> MAFSRPGLPVEYLQVPSASMGRDIKVQFQGGGPHAVYLLDGLRAQDDYNGWDINTPAFEE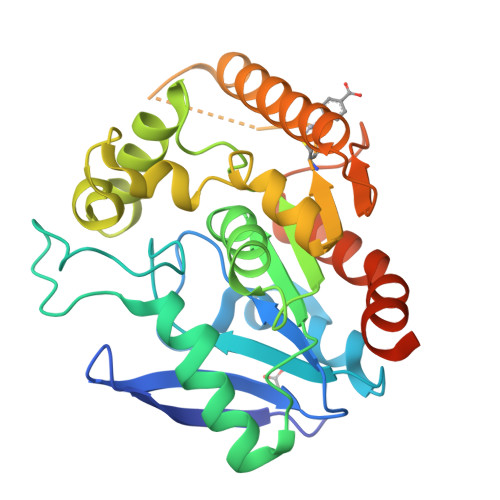YYQSGLSVIMPVGGQSSFYTDWYQPSQSNGQNYTYKWETFLTREMPAWLQANKGVSPTGNAAVGLSMSGGSALILAAYYPQQFPYAASLSGFLNPSEGWWPTLIGLAMNDSGGYNANSMWGPSSDPAWKRNDPMVQIPRLVANNTRIWVYXGNGTPSDLGGDNIPAKFLEGLTLRTNQTFRDTYAADGGRNGVFNFPPNGTHSWPYWNEQLVAMKADIQHVLNGATPPAAPAAPAAHHHHHH> MSILHTVNKSPFERNSLESCLKFATEGASVLLFEDGIYAALAGTRVESQVTEALGKLKLY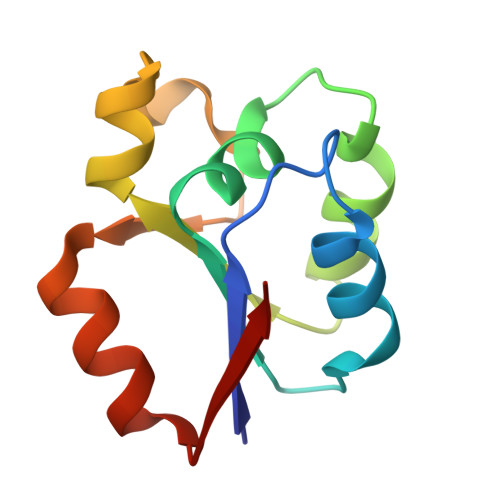VLGPDLKARGFSDERVIPGISVVDYAGFVDLTTECDTVQAWL>MSKTIATENAPAAIGPYVQGVDLGNMIITSGQIPVNPKTGEVPADVAAQARQSLDNVKAIVEAAGLKVGDIVKTTVFVKDLNDFATVNATYEAF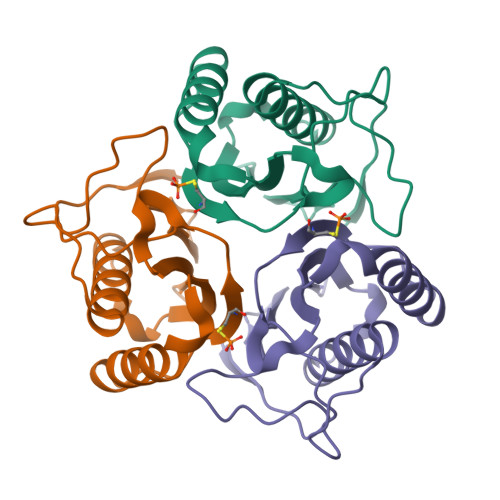FTEHNATFPARSCVEVARLPKDVKIEIEAIAVRR[3x]>[4x]GAMGMNGQGATSIPGEVAEQAMHWHLELQEPAVS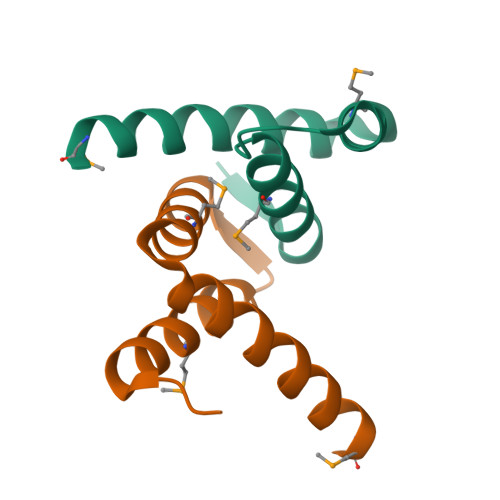AATLAACMSWRQAHPLHEHAWQRTQVFAQRLREMRSPGQRPLAHAALRPQQS> MGHHHHHHGSTFFNPDREGWLLKLGGGRVKTWKRRWFILTDNCLYYFEYTTDKEPRGIIPLENLSIREVEDPRKPN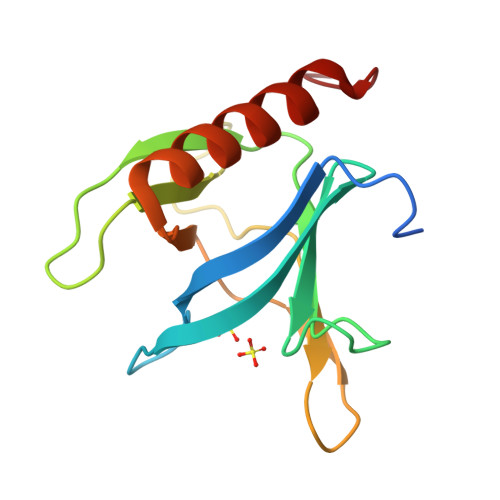CFELYNPSHKGQVIKACKTEADGRVVEGNHVVYRISAPSPEEKEEWMKSIKASISRDPFYDM> NTGDNSVCTTKTSTRIVGGTESSWGEWPWQVSLQVKLTAQRHLCGGSLIGHQWVLTAAHCFDGLPLQDVWRIYSGILELSDITKDTPFSQIKEIIIHQNYKVSEGNHDIALIKLQAPLEYTEFQKPISLPSKGDTSTIYTNCWVTGWGFSKEKGEIQNILQKVNIPLVTNEECQKRYQDYK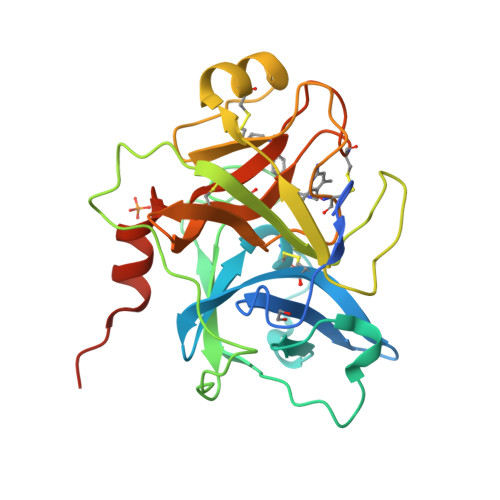ITQRMVCAGYKEGGKDACKGDSGGPLVCKHNGMWRLVGITSWGEGCARREQPGVYTKVAEYMDWILEKTQSSDGKAQMQSPA>[2x]MHHHHHHAAGIPMNNPAIKRIGNHITKSPEDKREYRGLELANGIKVLLISDPTTDKSSAALDVHIGSLSDPPNIAGLSHFLQHMLFLGTKKYPKENEYSQFLSEHAGSSNAFTSGEHTNYYFDVSHEHLEGALDRFAQFFLSPLFDESAKDREVNAVDSEHEKNVMNDAWRLFQLEKATGNPKHPFSKFGTGNKYTLETRPNQEGIDVRQELLKFHSAYYSSNLMAVVVLGRESLDDLTNLVVKLFSEVENKNVPLPEFPEHPFQEEHLKQLYKIVPIKDIRNLYVTFPIPDLQKYYKSNPGHYLGHLIGHEGPGSLLSELKSKGWVNTLVGGQKEGARGFMFFIINVDLTEEGLLHVEDIILHMFQYIQKLRAEGPQEWVFQELKDLNAVAFRFKDKERPRGYTSKIAGILHYYPLEEVLTAEYLLEEFRPDLIEMVLDKLRPENVRVAIVSKSFEGKTDRTEEWYGTQYKQEAIPDEVIKKWQNADLNGKFKLPTKNEFIPTNFEILPLEKEATPYPALIKDTAMSKLWFKQDDKFFLPKANLNFE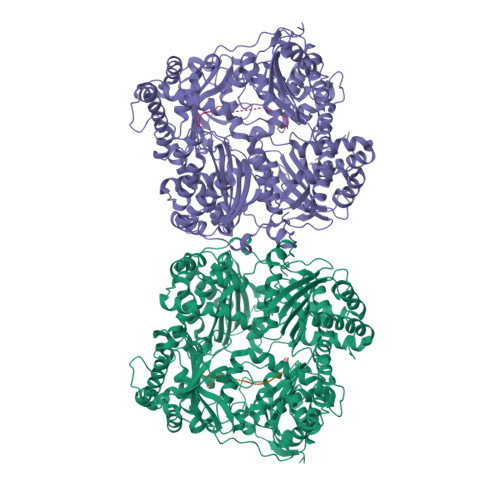FFSPFAYVDPLHSNMAYLYLELLKDSLNEYAYAAELAGLSYDLQNTIYGMYLSVKGYNDKQPILLKKIIEKMATFEIDEKRFEIIKEAYMRSLNNFRAEQPHQHAMYYLRLLMTEVAWTKDELKEALDDVTLPRLKAFIPQLLSRLHIEALLHGNITKQAALGIMQMVEDTLIEHAHTKPLLPSQLVRYREVQLPDRGWFVYQQRNEVHNNSGIEIYYQTDMQSTSENMFLELFAQIISEPAFNTLRTKEQLGYIVFSGPRRANGIQGLRFIIQSEKPPHYLESRVEAFLITMEKSIEDMTEEAFQKHIQALAIRRLDKPKKLSAESAKYWGEIISQQYNFDRDNTEVAYLKTLTKEDIIKFYKEMLAVDAPRRHKVSVHVLAREMDSNPVVGEFPAQNDINLSQAPALPQPEVIQNMTEFKRGLPLFPLVKPHINFMAAKL;>ASLAADTPTACCFSYTSRQIPQNFIADYFETSSQCSKPGVIFLTKRSRQVCADPSEEWVQKYVSDLELSA[2x]> FMVSLPRMVYPQPKVLTPCRKDVLVVTPWLAPIVWEGTFNIDILNEQFRLQNTTIGLTVFAIKKYVAFLKLFLETAEKHFMVGHRVHYYVFTDQPAAVPRVTLGTGRQLSVLEVRAYKRWQDVSMRRMEMISDFCERRFLSEVDYLVCVDVDMEFRDHVGVEILTPLFGTLHPGFYGSSREAFTYERRPQSQAYIPKDEGDFYYMGAFFGGSVQEVQRLTRACHQAMMVDQANGIEAVWHDESHLNKYLLRH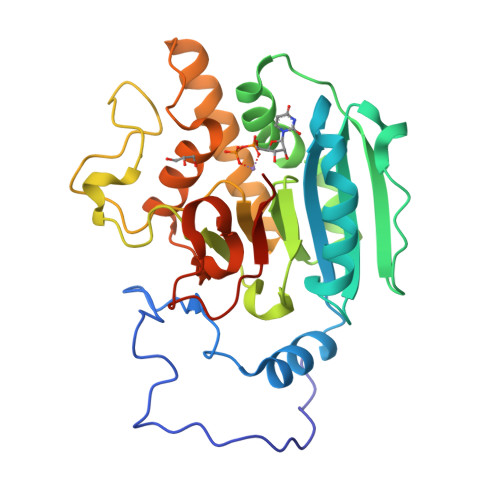KPTKVLSPEYLWDQQLLGWPAVLRKLRFTAVPKNHQAVRNPE> HMPREPVTPDSDHPDPVETVRQLTAHVLGLTAAADVEMTRSFKDLGFDSLMSVELRDRLCAATGLSLAT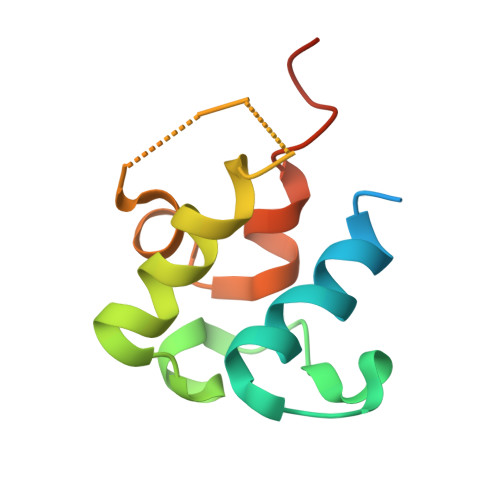TLLYDHPSPAETAEFVRARLTGDEA>[2x]SEKITDGINKTISATGNIYNISSANELNALKLQPGDKVIFKKGNWKNQQINFKANGTKEKPVVLAAEKGGETIFSGNSNLKIDGNWLVVDGFVFKDGFSEKADVILFTKSTSNSRITNSSIINYNHPDKTFDYKWLSLNGENNRVDHCDFTGKTHQGTTLVVWL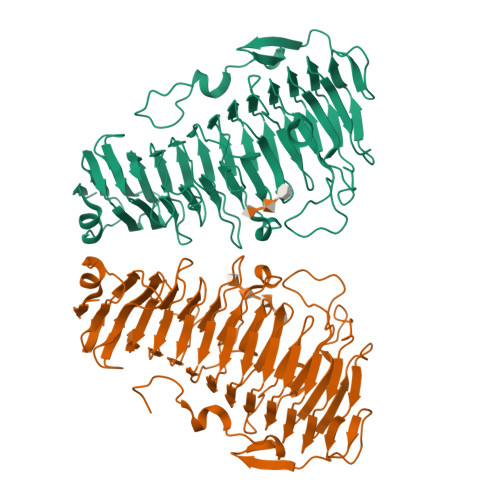DEKPNHHQIDHNYFGPRPALGVNGGETIRIGTSTWSMHDSYTLVENNIFDKCDGEMEIISLKSGHNTVNNNLFYECDGTVTFRHGNYNTVSNNYILGNGKKNTGGIRIIGENHKVFGNYLQGLDGSGLRAAISIMSALEKPQLHEYFQVINPQIVGNIIADSKEGIDIGAGKNEKRMLPPKDGFLKNNYVINTRTVIKTENEPEGLLIENNQTDASSLPKGFTKVGSDLVKSDGIWQKKNDVKTPFWKKEKIGPEWNNVKMN>[4x]MGILALVTDAVSLPIDYDMPPLLEACRTVGITAEVCDWEDGTVDWSRFEAVVFRSPWTWAERQAEFLAFCERVSHVTRLITPMPLVRWALDKRYLADLAAHGVPVIPTTVVAPGSDALAAVRDFLAA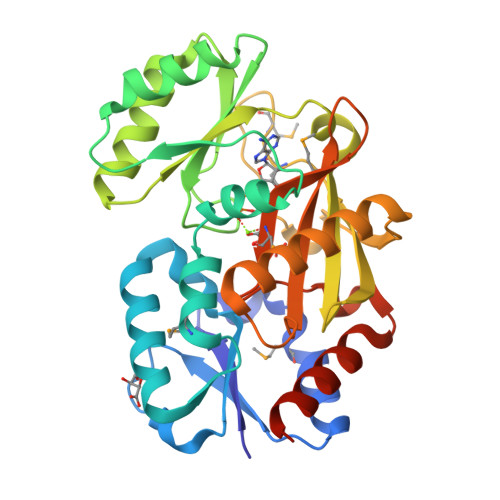RPEAREFVVKPTDGCYSKDVQRYQRSLAEPASRHVARLLANGSHVILQPYVESVDRHGETDLTFFDGVYSHAIHKGAMLMPDGTVHVPTLDFRQARDADEDQRAVAAAALAASVAHLGLDLPLVCGRVDLVRGADGSPMVLEMELCEPSLNLTFSEDGALRFAQALAERLKPLEHHHHHH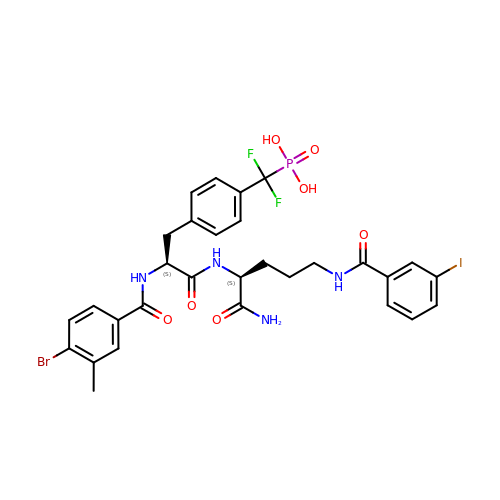N-(4-bromo-3-methylbenzoyl)-4-[difluoro(phosphono)methyl]-L-phenylalanyl-N~5~-(3-iodobenzoyl)-L-ornithinamide | C30 H31 Br F2 I N4 O7 P | PSWNGHKKMCDZPT-DQEYMECFSA-N> RSPWCVICDPSVVLALKSLEKDYLPGHLDAKHHKAMMERVENAVKDFQELSLNEDAYMGVVDEATLQKGSWSLLKDLKRITDSDVKGDLFVKELFWMLHLQKETFATYVARFQKEAYCPNKCGVMLQTLIWCKNCKKE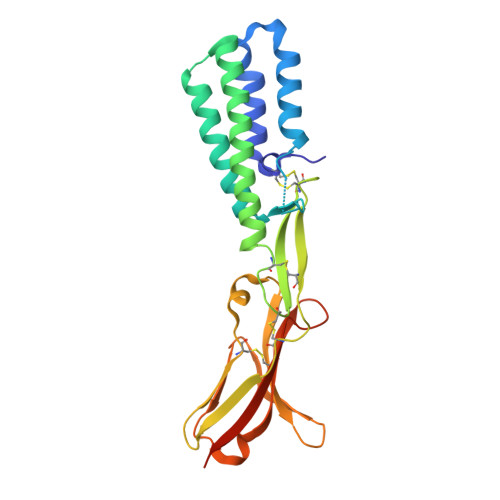VHACRKSYDCGERNVEVPQMEDMILDCELNWHQASEGLTDYSFYRVWGNNTETLVSKGKEATLTKPMVGPEDAGSYRCELGSVNSSPATIINFHVTVLPKEFLEVLFQ>[2x]MGHHHHHHMKLRGKTAVVTGGAGGIGRAVTRVFVREGARVLFVDVDDDRGRALESELTGAGGEAKFLQADISRRESADQIRDAAVAAFGGIDILVNNAHASRQALLVEHTPEMFELSFGTGFYPTVHLMQACYPQLKQARGSVVNFGSGSALDGMPTQTSYAAAKEAIRAVSRVAANEWAADGIRVNVVCPFAATEGVQAWQQAFPDRAAAAAAKVPLQRIGDPETDIAPVVVFLASDD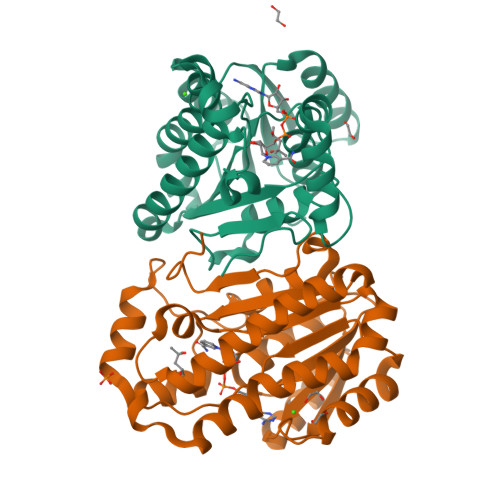SKYMTGQTLMADGGSIKLR>KIKACIDEVTTTLEETKFLTNKLLLFADINGKLYHDSQNMLRGEDMSFLEKDAPYMVGDVITSGDITCVVIPSKKAGGTTEMLSRALKKVPVDEYITTYPGQGCAGYTLEEAKTALKKCKSAFYVLPSEAPNAKEEILGTVSWNLREMLAHAEETRKLMPICMDVRAIMATIQRKYKGIK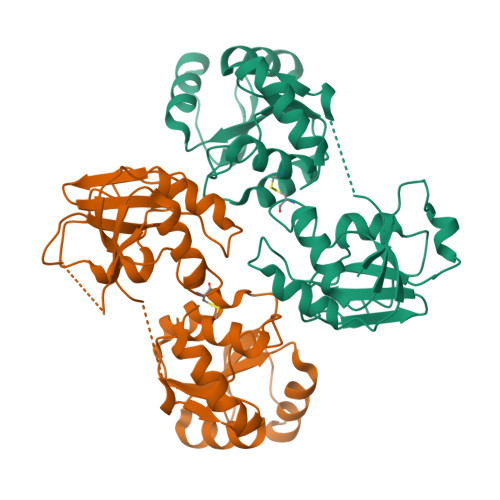IQEGIVDYGVRFFFYTSKEPVASIITKLNSLNEPLVTMPIGYVTHGFNLEEAARCMRSLRAPAVVSVSSPDAVTTYNGYLTSSS[4x]> MTFKAPDSLAEQIAHHLAERIIRGELKERERIQEQKVTQTLNVSRGSVREALLILERRHLVNILPRRGAQVSELSPQHVESLYALIVQLYILLAESVARRWRSEAELAPFLVIQQRLLNNL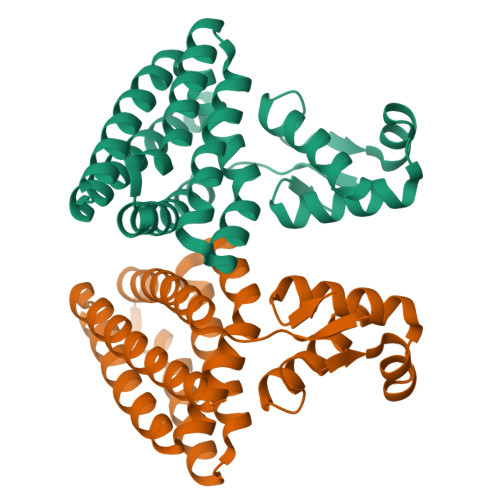AQSDIDGFVEASFDIMRAAFPFANNPYLQETVENLLPAVSRAYHLALERRKAEMNQFLGSFAQLLQAVIARDEARIREVLLEYGRHNCQLVLAALAER>[2x]MAKTY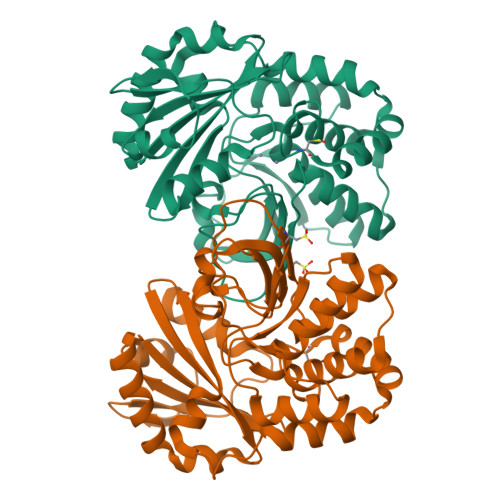IFGHKNPDTDAISSAIIMAEFEQLRGNSGAKAYRLGDVSAETQFALDTFNVPAPELLTDDLDGQDVILVDHNEFQQSSDTIASATIKHVIDHHRIANFETAGPLCYRAEPVGCTATILYKMFRERGFEIKPEIAGLMLSAIISDSLLFKSPTCTQQDVKAAEELKDIAKVDIQKYGLDMLKAGASTTDKSVEFLLNMDAKSFTMGDYVTRIAQVNAVDLDEVLNRKEDLEKEMLAVSAQEKYDLFVLVVTDIINSDSKILVVGAEKDKVGEAFNVQLEDDMAFLSGVVSRKKQIVPQITEALTKLEHHHHHH>[8x]SNAMTIVQAAQSRYSTKAFDASRKLPEEKVAAVKELIRMSASSVNSQPWHFIVASSEEGKARIAKATQGGFAFNERKILDASHVV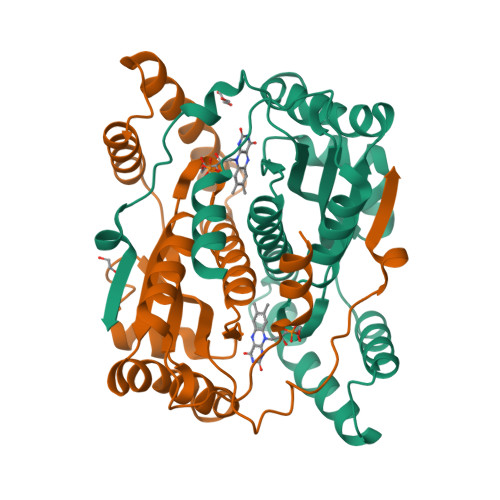VFCAKTAIDEAYLLDLLESEDKDGRFADVEAKNGMHAGRSFFVNMHRFDLKDAHHWMEKQVYLNVGTLLLGASAMEIDAVPIEGFDAKVLDEEFGLREKGFTSVVIVPLGYHSEDDFNAKLPKSRWSAETVFTEI>[3x]MGDTKEQRILRYVQQHAKPGDPQSVLEAIDTYCTQKEWAMNVGDAKGQIMDEVIQEHNPSLVLELGAYCGYSAVRMARLLSPGARLLTMEK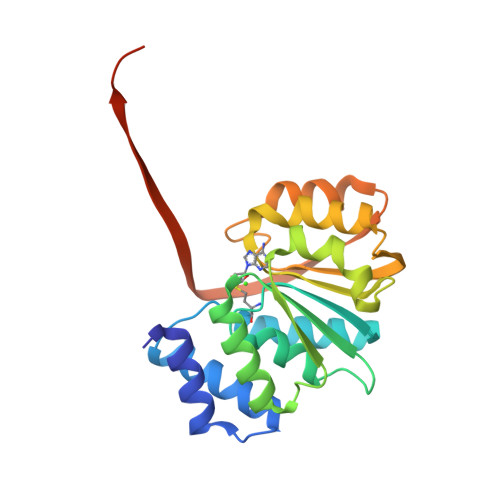NPDYAAITQQMLNFAGLQDKVTILIGASQDLIPQLKKYDVDTLDMVFLDHWKDRYLPDTILLEECGLLRKGTVLLADNVIVPGTPDFLAYVRGSSSFECTHYSSYLEYMKVVDGLEKAVYKGPSSPKQPLEHHHHHH>MWGKKDAGTELTNYQTLATNTIGMMKGVDGYAFTSGAKMTDTLIQAGAAKGMTVSGDPASGSATLWNSWGGQIVVAPDTAGGTGFNNGFTITTNKVPQSACVSISTGMSRSGGTSGIKI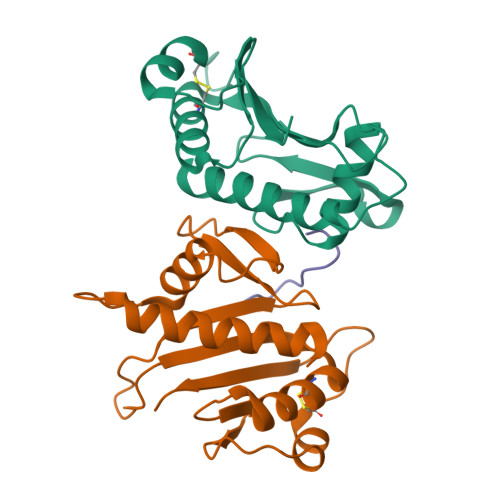NGNNHTDAKVTAEIASSECTADNGRTGTNTLVFNYNG[2x];> SYDPDNKEER>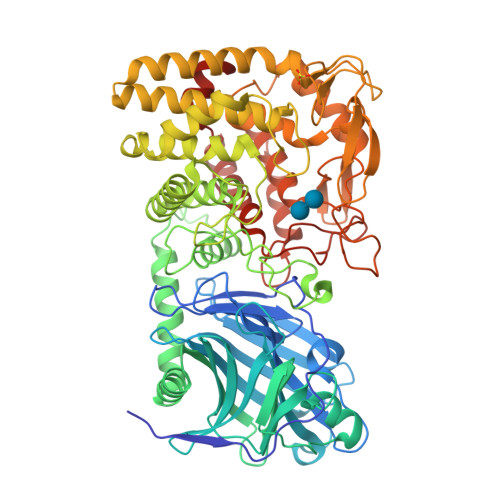[2x]VLSGCSNNVSSIKIDRFNNISAVNGPGEEDTWASAQKQGVGTANNYVSKVWFTLANGAISEVYYPTIDTADVKEIKFIVTDGKSFVPDETKDAISKVEKFTDKSLGYKLVNTDKKGRYRITKDIFTDVKRNSLIMKAKFEALEGSIHDYKLYLAYDPHIKNQGSYNEGYVIKANNNEMLMAKRDNVYTALSSNIGWKGYSIGYYKVNDIMTDLDENKQMTKHYDSARGNIIEGAEIDLTKNSEFEIVLSFGQSDSEAAKTALETLGEDYNNLKNNYIDEWTKYCNTLNNFNGKANSLYYNSMMILKASEDKTNKGAYIASLSIPWGDGQRDDNTGGYHLVWSRDLYHVANAFIAAGDVDSANRSLDYLAKVVKDNGMIPQNTWISGKPYWTGIQLDEQADPIILSYRLKRYDLYDSLVKPLADFIIKIGPKTGQERWEEIGGYSPATMAAEVAGLTCAAYIAEQNKDYESAQKYQEKADNWQKLIDNLTYTENGPLGNGQYYIRIAGLSDPDADFMINIANGGGVYDQKEIVDPSFLELVRLGVKSADDPKILNTLKVVDSTIKVDTPKGPSWYRYNHDGYGEPSKTELYHGAGKGRLWPLLTGERGMYEIAAGKDATPYVKAMEKFANEGGIISEQVWEDTGLPTDSASPLNWAHAEYVILFASNIEHKVLDMPDIVYKRYVA> GPLGSNRKRLPSYLKPGSAVEI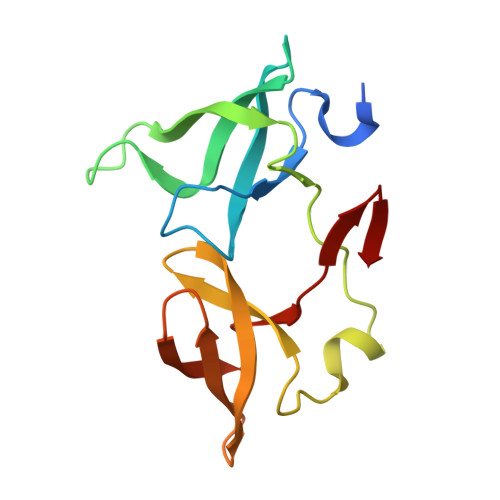SSDEIGFRGSWYMGKVITIPSSSDKDSVKCQVEYTTLFFDKEGTKPLKEVVDMSQLRPPAPPMSEIEKKKKIVVGEEVDAFYNDGWWEGDVTEVLDDGKFSVFFRSSKEQIRFRKDELRFHREWVDGAWK> GSMKTNLKGETALHRACINNQVEKLILLLSLPGIDINVKDNAGWTPLHEACNYGNTVCVQEILQRCPEVDLLTQVDGVTPLHDAL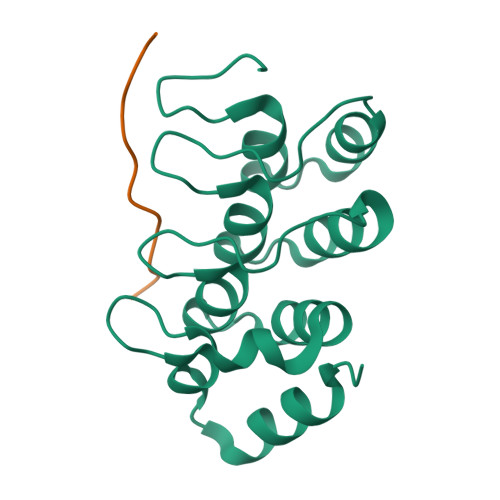SNGHVEIGKLLLQHGGPVLLQQRNAKGELPLDYVVSPQIKEELFAITKIED;> GLGKGGAKRHRKVLRDN6-[4-[6-[(4,4-dimethylpiperidin-1-yl)methyl]pyridin-3-yl]-1-oxa-4,9-diazaspiro[5.5]undecan-9-yl]-N-(phenylmethyl)pyrimidin-4-amine 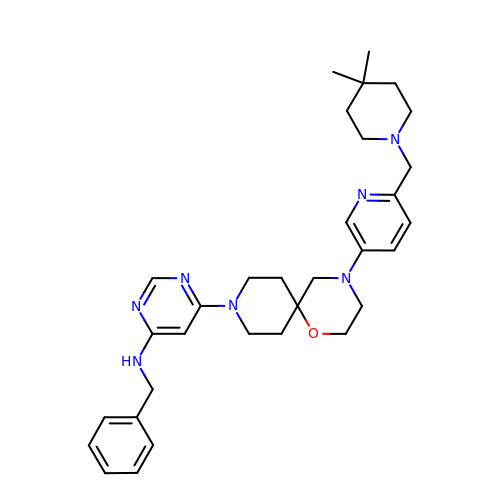| C32 H43 N7 O | RJEWLHZZXYDBNT-UHFFFAOYSA-N Neisseria gonorrhoeae responds to host-derived antimicrobials by inducing the expression of the mtrCDE-encoded multidrug efflux pump, which expels microbicides, such as bile salts, fatty acids, and multiple extrinsically administered drugs, from the cell. The mtrCDE genes are organized in a three-gene operon, and their expression is repressed by the divergently transcribed transcription regulator MtrR, which is a dimeric TetR family member with a predicted N-terminal helix-turn-helix (HTH) DNA binding motif and a C-terminal dimerization/inducer-binding domain. Under physiological conditions, MtrR binds to a 27-bp direct repeat located upstream of the mtrC transcription start site in the intergenic region between the mtrC and mtrR genes and represses mtrCDE transcription, as well as that of its own gene. As in other bacterial multidrug-binding regulators, MtrR likely responds to the influx of multiple cytotoxins into the cytoplasm by dissociating from the mtrC promoter and relieving repression of mtrCDE gene expression.

The native structure was refined to 2.0-Å resolution with final Rwork and Rfree values of 20.4% and 24.7%, respectively. The asymmetric unit contains two MtrR dimers, with nearly all 210 residues of each protomer observed, with the exception of residues 1 through 7 in two subunits or 1 through 8 in the other subunits. The subunits of each dimer are composed of nine α helices. MtrR has two distinguishable functional domains: an N-terminal DNA binding domain with a helix-turn-helix (HTH) motif and a C-terminal dimerization/ligand-binding domain. The dimer interface is formed primarily by the burial of hydrophobic residues in the middle of a four-helix bundle that is formed by α8 and α9 of each subunit. As observed in all other TetR family members, the multidrug-binding pocket of MtrR is located in the C-terminal domain with ligand-binding residues contributed from all C-terminal helices except α9. The initial solvent-flattened electron density map revealed positive electron density in each of the four independent putative ligand-binding pockets of each MtrR protomer, suggesting a “ligand” was fortuitously captured during the purification or crystallization process. The density could be fit by CAPS, the biological buffer component of the MtrR crystallization reagent. Thus, our final structural model of MtrR does not contain CAPS. Despite our inability to refine this mystery electron density with CAPS, its location provided insight into the chemical makeup of the putative MtrR binding pocket. This cavity is primarily composed of nonpolar residues and is populated with more than 20 hydrophobic or aromatic amino acid residues.

>[4x]MRKTKTEALKTKEHLMLAALETFYRKGIARTSLNEIAQAAGVTRGALYWHFKNKEDLFDALFQRICDDIENCIAQDAADAEGGSWTVFRHTLLHFFERLQSNDIHYKFHNILFLKCEHTEQNAAVIAIARKHQAIWREKITAVLTEAVENQDLADDLDKETAVIFIKSTLDGLIWRWFSSGESFDLGKTAPRIIGIMMDNLENHPCLRRK> SLAADTPTACCFSYTSRQIPQNFIADYFETSSQCSKPGVIFLTKRSRQVC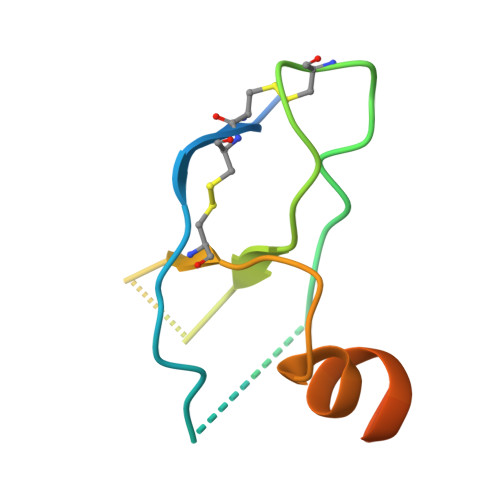ADPSEEWVQKYVSDLELSAHHHHHH>[4x]MAHHHHHHMNALEHQLDYPFADTLPAAGDTFEVAPGVRWLRMPLPFSLDHINLWLLRDEIDGQAGWTIVDCGISSEAIRTHWEQIFDRHLDGLPVLRVLVTHCHPDHFGLANWLCEGGDQGRWNVRLWMTLGEYMFGCLMAAGNGSNAGGAAAADHFARHGLTDPAALDKLRSRRSYYSDLVP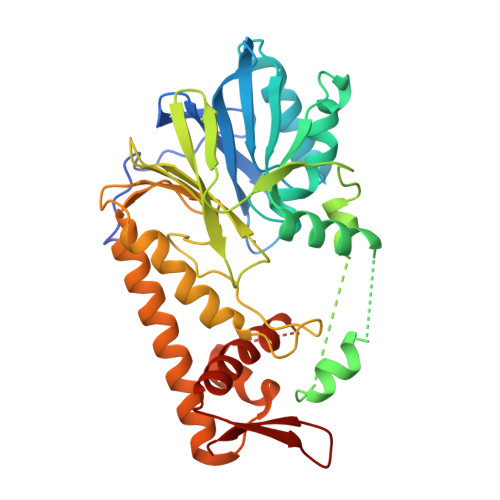AVPPRYRRLREGDAVKIGARTWRVVTGYGHSPEHCALHSEADGVLISGDMVLPRISTNVSVFDLEPEANPLALYLESLGRYETMAPDTLVLPSHGKPFRGVRTRIAQLRAHHDARLEEVRVACAEKPMSAAGIVPIMFRRRELDIHQMTFALGEALAHLNLLWLAGELVREHGDDGVIRYARA> AAPNDPSYRQQWHYFSNYGVKADKVWDRGFTGQGVVVSVVDTGILDHVDLNGNMLPGYDFISSAPKARDGDQRDNNPADEGDWFDNWDCGGYPDPRREKRFSTWHGSHVAGTIAAVTNNGVGVAGVAYGAKVIPVRVLGKCGGYDSDITDGMYWSAGGHIDGVPDNQNPAQVINMSLGGDGDCSQSSQRIIDKTTNLGALIVIAAGNENQDASRTWPSSCNNVLSVGATT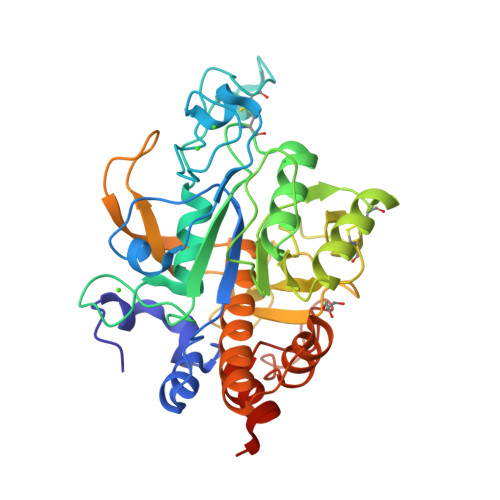PKGKRAPFSNYGARVHLAAPGTNILSTIDVGQAGPVRSSYGMKAGTSMAAPHVSGVAALVISAANSIGKTLTPSELSDILVRTTSRFNGRLDRGLGSGIVDANAAVNAVLGDQNLEHHHHHH> DQYEYKYPAIKDLKKPCITLGKAPDLNKAYKSVLSGMNAAKLDPDDVCSYLAAAMQFFEGTCPEDWTSYGILIARKGDRITPNSLVEIKRTDVEGNWALTGGMELTRDPTVSEHASLVGLLLSLYRLSKISGQNTGNYKTNIADRIEQIFETAPFVKIVEHHTLMTTHKMCANWSTIPNFRFLAGTYDMFFSRIEHLYSAIRVGTVVTAYEDCSGLVSFTGFIKQINLTAREAILYFFHKNFEEEIRRMFEPGQETAVPHSYFIHFRSLGLSGKSPYSSNAVGHVFNLIHFVGCYMGQVRSLNATVIAACAPHEMSVLGGYLGEEFFGKGTFERRFFRDEKELQEYEAAELTKSDVALADDGTVNSDDEDYFSGETRSPEAVYTRIMMNGGRLKRSHIRRYVSVSSNHQARPNSFAEFLNKTYSNDS;> MSKIFVNPSAIRAGLADLEMAEETVDLINRNIEDNQAHLQGEPIEVDNLPEDMGRLHLDGGKSPNPGELEHHHHHH

As for all non-segmented negative RNA viruses, rabies virus has its genome packaged in a linear assembly of nucleoprotein (N), named nucleocapsid. RABV N is composed of two globular domains that are connected by a hinge, creating an RNA binding groove. It also comprises two subdomains, an N-terminal extension, named the NNT-ARM, and an internal loop in the C-terminal domain, named the NCT-ARM, that dock to neighboring subunits in the polymeric form and thereby stabilize the assembled NC. Thus, genome replication requires the production of the unassembled RNA-free N protein, named N0, in the form a complex named the N0−P complex, in which P prevents the polymerization of N and the illegitimate assembly with cellular RNA until N is transferred to nascent viral RNA.

In this study, we reconstituted a soluble heterodimeric complex between an armless N protein of rabies virus (RABV), lacking its N-terminal subdomain (NNT-ARM), and a peptide encompassing the N0 chaperon module of the P protein. The NΔ230−P68 complex crystallized with a single molecule in the asymmetric unit and the crystals diffracted up to 2.3 Å resolution. The NΔ230−P68 complex contained no RNA and an analysis with the webserver PDBePISA revealed no intermolecular interactions between neighboring heterodimers besides the crystal contacts (Complex Formation Significance Score (CSS) = 1.0 for the interaction between NΔ230 and P68 and CSS = 0.0 for all other contacts), demonstrating the absence of N polymerization in the crystal. In the absence of neighboring N subunits, the entire NCT-ARM (aa 350–400) was not visible in the crystal structure and a 5-residue loop in NNTD (aa 155–159) was also absent from the crystal structure, suggesting that it was flexible in the absence of RNA as expected, since this loop interacted with one of the bound nucleotides in the N−RNA complex. Two parts of P68 were clearly visible in the electronic density; residues from 4 to 15 were bound in a groove of NCTD with residues from 9 to 12 forming a helical turn, while residues from 20 to 39 formed a long α helix that docked at the interface between NNTD and NCTD. The binding of the P68 N-terminal moiety involved three H-bonds and four salt-bridges and buried a surface area of 1190 Å2, whereas the binding of the P68 C-terminal moiety involved thirteen H-bonds and three salt bridges and buried a surface area of 1617 Å2. As in other Mononegavirales N0−P complexes, the P chaperone module prevented the polymerization of N by interfering with the binding of the NNT-ARM and NCT-ARM subdomains from adjacent N subunits. The N-terminal part of RABV P68 competed with the NCT-ARM of the Ni+1 protomer, whereas the C-terminal part competed with the NNT-ARM of the Ni–1 protomer. Additionally, in the RABV NΔ230−P68 complex, the RNA binding groove in the N protein adopted a close conformation as in the N−RNA complex and in VSV NΔ210−P60 structure.> MLNIGDLLGSTPAKDQGCSRTCESQFCTIAPLLRYGKYCGILYSGCPGERPCDALDACCMVHDHCVDTHNDDYLNTMCNENLLSCID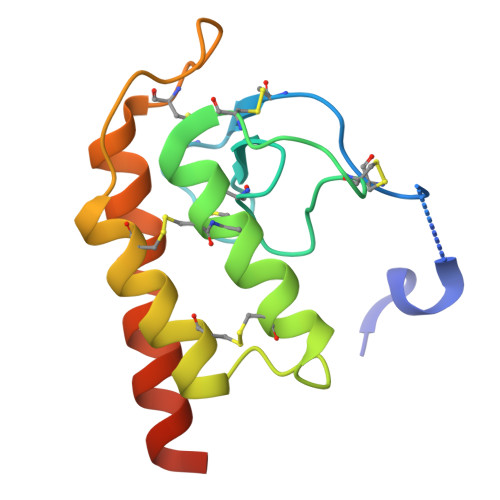RVSGATFPGNKCNVGQTASVIRGVIETAVFAGKILHKRDDGQ>GSPKDPKRIAVVAPTYAGGLKKLGANIVAVNQQVDQSKVLKDKFKGVTKIGDGDVEKVAKEKPDLIIVYSTDKDIAAYQAVAPTVVVDYNKHKYLEQQEMLGKIVGKEDKVKAWKKDWEETTAKDGKEIKKAIGQDATVSLFDEFDKKLYTYGDNWGRGGEVLYQAFGLKMQ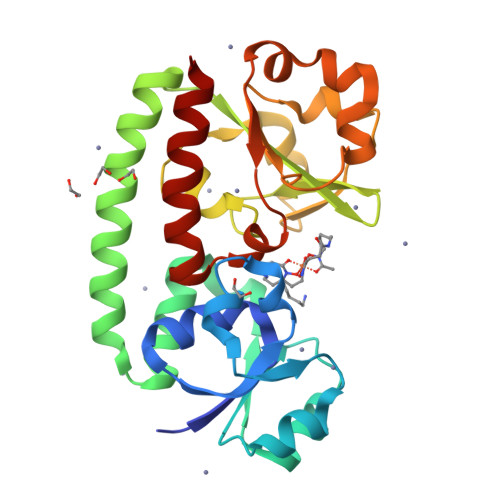PEQQKLTAKAGWAEVKQEEIEKYAGDYIVSTSEGKPTPGYESTNMWKNLKATKEGHIVKVDAGTYWYNDPYTLDFMRKDLKEKLIKAAK[4x]>[2x]MIKATYSSAKDFYSLLSGLLKVTDEIILNFTEDSIFSRYLTDDKVLMVIFKIPKEYLEDYTIDKPLGIKINI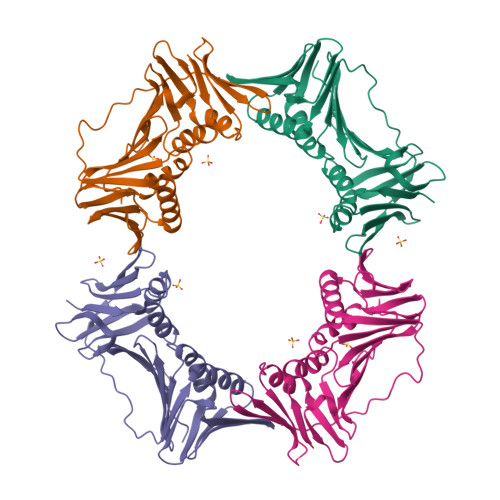NDLKKILGKAKSKSATVTLEETEAGLKVTVRDEKTGTRSNIYIKGEKTSIDQLTEPKVNLSVTFTTDGDVLKDIARDLSLVGEEVEISADENTVTLSTEEAGRTYKSLLKQDKPLKSLNVESPSKAVYSIEVLKDVFKVTSISQNVTVGFGNNIPMKIEVPTDSGGQLIFWIAPRL;>MRVKVIDADAFSYIFRTLEEFIDEITLDFTSDGLKIRGIDPSRVTFIDILIPAGYFEEYNVEKEEKVGVKLEDFTDVLKTVTKNDSLYLETDENQNIKVTLDGVYERTFTFPSIVASEIETPNLNLEFPFKAKALTVTFTDIIDEIEDIGGDSITFKAEGGKLYLSANSDMGSSTIELSTENGGLLESEGGDAESVYGLEYVVNTSKMRKPSDTVEIAFGSQIPLKLRYNLPQGGYADFYIAPRAE[2x]> GPMGNGMNKILPGLYIGNFKDARDAEQLSKNKVTHILSVHDSARPMLEGVKYLCIPAADSPSQ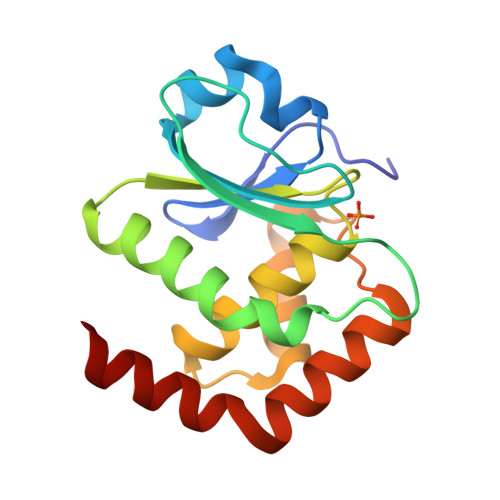NLTRHFKESIKFIHECRLRGESCLVHSLAGVNRSVTLVIAYIMTVTDFGWEDALHTVRAGRSCANPNVGFQRQLQEFEKHEVHQYRQWLKEEYG>[4x]AAGVAFQGAVQVHVVDHPLAAARLTTLRDERTDNAGFRAALRELTLLLIYEAT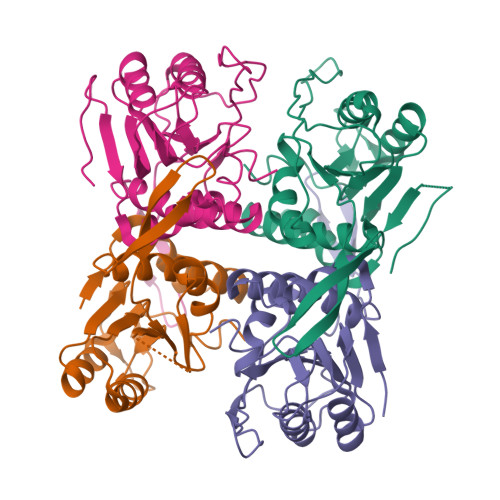RDAPCEPVPIRTPLAETVGSRLTKPPLLVPVLRAGLGMVDEAHAALPEAHVGFVGVARDEQTHQPVPYLDSLPDDLTDVPVMVLDPMVATGGSMTHTLGLLISRGAADITVLCVVAAPEGIAALQKAAPNVRLFTAAIDEGLNEVAYIVPGLGDAGDRQFGPR>VSIYDPAAADRAEEERIERWVEQLREALVGDGFLLHYQPVLNLQGEPLELYQAFLRLERNGEMMSPNAFMAIAEEHDLVTEIDRWVVARAIRQLGERQRAGHKTHLLVRIGPNSFSDPQMIDTIREQLAVYGVPGERLWLQTPESKVFTHLRNAQQFLAAVSAMDCKVGLEQFGSGLDSFQLLAHFHPAFLKLDRGITGDIASARDSQEKIREITSRAQPAGILTMAEFVADAQSMSSFFSAGVDYVQGDFVAPTGPLMNYEFG[2x];>MSAMNARQGILSLALKDKPALYSAYM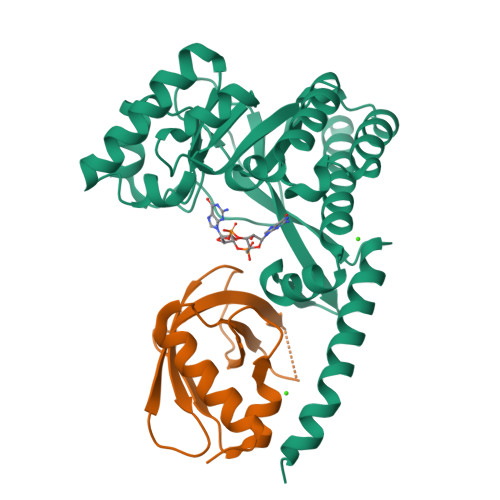PFVKGGGIFVPTPKRYMLGDEVFLLLTLPDSSERLPVAGKVIWTTPAGAQGNRAAGIGVQFPDGPEGEAVRNKIETLLAGLTTSDKPTHTM[2x]>[2x]ARSLLPLSTSLDHRSKEELHQDCLVLATAKHSRELNEDVSADVEERFHLGLFTDRATLYRMIDIEGKGHLENGHPELFHQLMLWKGDLKGVLQTAAERGELTDNLVAMAPAAGYHVWLWAVEAFAKQLCFQDQYVKAASHLLSIHKVYEAVELLKSNHFYREAIAIAKARLRPEDPVLKDLYLSWG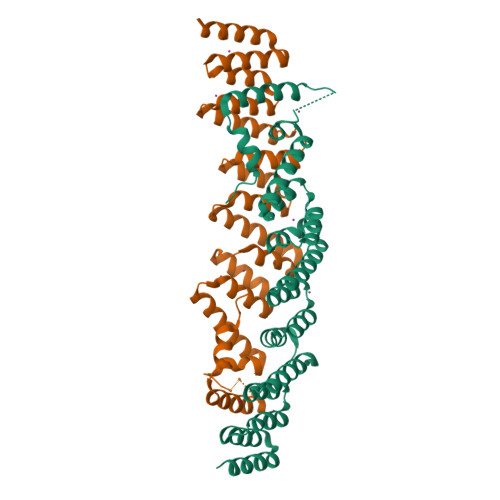TVLERDGHYAVAAKCYLGATCAYDAAKVLAKKGDAASLRTAAELAAIVGEDELSASLALRCAQELL> AEAGITGTWYNQLGSTFIVTAGADGALTGTYESAVGNAESRYVLTGRYDSAPATDGSGTALGWTVAWKNNYRNAHSATTWSGQYVGGAEARINTQWLLTS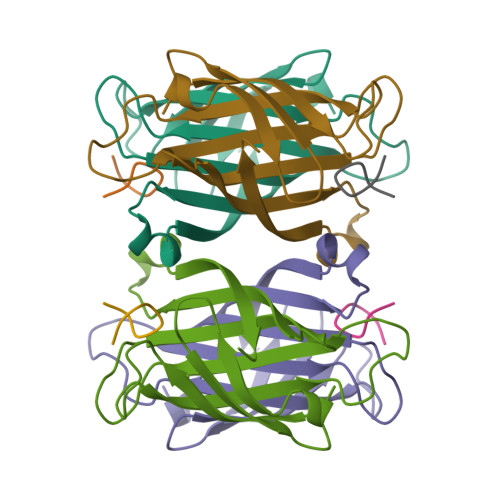GTTEANAWKSTLVGHDTFTKVKP;> XCHPQGPPCX FKBP12 proteins are members of the FKBP PPIase (peptidyl-prolyl isomerase) superfamily and catalyze the cis-trans isomerization of proline imidic peptide bonds. The immunosuppressants first bind to their respective immunophilins, FKBP12 (12-kDa FK506 binding protein) and CypA (cyclophilin A), which subsequently bind to calcineurin in a groove between the CnA and CnB subunits. The immunophilin-immunosuppressant complexes inhibit calcineurin serine-threonine phosphatase activity, blocking the dephosphorylation of downstream targets, such as the human nuclear transcription factor NFAT (nuclear factor of activated T cells), involved in T-cell activation and interleukin-2 transcription, and the fungal transcription factor Crz1 (NFAT homolog), implicated in virulence, stress response, and thermotolerance. To this end, we characterized high-resolution structures of the Mucor circinelloides FKBP12 bound to FK506 and of the Aspergillus fumigatus, M. circinelloides, and human FKBP12 proteins bound to the FK506 analog APX879, which exhibits enhanced selectivity for fungal pathogens.

McFKBP12 shares 58% and 65% sequence identity with hFKBP12 and AfFKBP12, respectively. To correlate sequence variations with structure and identify potential differences between McFKBP12 and other FKBP12 proteins, we attempted to crystallize McFKBP12 in its apo form. All attempts failed to yield protein crystals, hinting at potentially high conformational flexibility of McFKBP12. However, crystals were obtained with the FK506-bound form (2.5 Å, P3221), suggesting rigidification of McFKBP12 by FK506 binding. McFKBP12 shares the same fold as hFKBP12 and AfFKBP12 (Cα-RMSD [root mean square deviation], ∼0.5 Å) with a 5-stranded β-sheet wrapping around an α-helix. The three main loops defining the FK506-binding cavity (40’s, 50’s, and 80’s loops) adopt the same conformation as observed in apo and FK506-bound forms of other FKBP12 proteins. When bound to McFKBP12, FK506 also adopts the same conformation as when bound to other mammalian and fungal FKBP12 proteins (FK506 RMSD, ∼0.3 Å). Six hydrogen bonds (H-bonds) between FK506 and McFKBP12 are observed: 2 involving the backbone of residues Gln55 and Ile57 and 4 to the side chains of residues Tyr27, Asp38, and Tyr83. Interestingly, in McFKBP12 residue 88 is a Tyr, potentially sterically hindering the ternary complex formation with A. fumigatus calcineurin. AfFKBP12 and McFKBP12 also interact tightly with FK506 (KD, 4.7 ± 0.6 and 3.0 ± 0.7 nM, respectively).

>GSHMGVTVERIAPGDGKNFPKKGDKVTIHYVGTLENGDKFDSSRDRGSPFQCTIGVGQVIKGWDEGVTQLSVGEKARLICTHDYAYGERGYPGLIPPKATLNFEVELIKIN[4x]> SMQEEDTFRELRIFLRNVTHRLAIDKRFRVFTKPVDPDEVPDYVTVIKQPMDLSSVISKIDLHKYLTVKDYLRDIDLICSNALEYNPDRDPGDRLIRHRACALRDTAYAIIKEELDEDFEQLCEEIQESR;> GLGKGGAY

All ATAD2 orthologs share a characteristic N-terminal AAA ATPase domain and a C-terminal bromodomain. Additional functional studies allowed us to characterize the normal function of Atad2, and to show that it is a general auxiliary factor targeting acetylated histones and facilitating chromatin-templated processes by maintaining chromatin accessible. However, in contrast to FACT, Atad2 bears a bromodomain capable of specifically guiding the protein toward acetylated histones where it could act as a molecular motor thanks to its AAA ATPase domain. To elucidate the structural basis of the ATAD2–histone interaction, we co-crystallized the ATAD2 bromodomain with peptides derived from the acetylated H4 tail.

We previously found the preference of ATAD2 bromodomain for multiple acetylated histone tails, and we had observed that mouse Atad2 preferentially binds to H4K5ac. Consequently, we focussed on H4 acetylated on K5 and K12. Hence, the purified ATAD2 bromodomain was crystallized with H4 tail peptides monoacetylated at either of these two sites. As described for other bromodomains, water molecules occupy the bottom of the acetyl-lysine binding site. For the two acetylated H4 peptides, residues R3 to G7 and G9 to G13 are well resolved in the electron density maps (lower left). However, apart from these conserved interactions, which are also shared with the binding mode of the isolated acetyl-lysine residue, the binding mode of the H4K5ac- and H4K12ac-containing peptides outside the central binding pocket is highly diverse. The H4K12ac-containing peptide forms only backbone or water-mediated interactions with the ATAD2 bromodomain, and the hydrophobic residue L10 adopts a seemingly unfavourable position next to a polar surface pocket (lower right).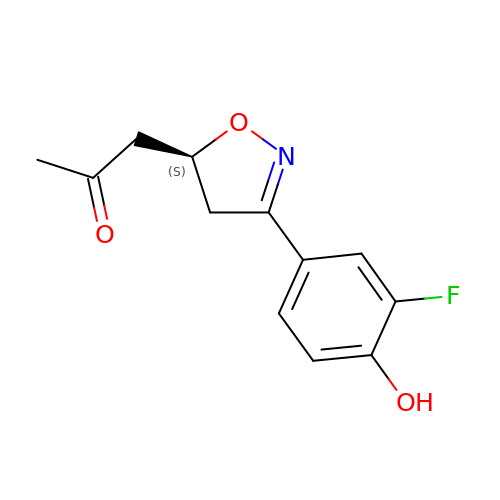1-[(5S)-3-(3-fluoro-4-hydroxyphenyl)-4,5-dihydro-1,2-oxazol-5-yl]propan-2-one | C12 H12 F N O3 | LDIXQWIEGSUIMD-SECBINFHSA-N> AYDRAITVFSPDGRLFQVEYALEAVKKGSTALGMKFANGVLLISDKKVRSRLIEQNSIEKIQLIDDYVAAVTSGLVADARVLVDFARISAQQEKVTYGSLVNIENLVKRVADQMQQYTQYGGVRPYGVSLIFAG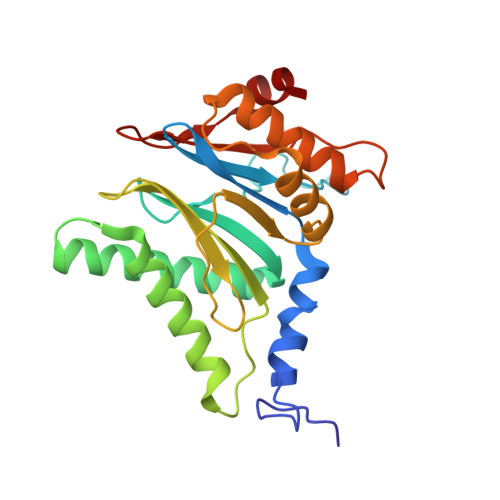IDQIGPRLFDCDPAGTINEYKATAIGSGKDAVVSFLEREYKENLPEKEAVTLGIKALKSSLEEGEELKAPEIASITVGNKYRIYDQEEVKKFL> ATFISVQLKKTSEVDLAKPLVKFIQQTYPSGGEEQAQYCRAAEELSKLRRAAVGRPLDKHEGALETLLRYYDQICSIEPKFPFSENQICLTFTWKDAFDKGSLFGGSVKLALASLGYEKSCVLFNCAALASQIAAEQNLDNDEGLKIAAKHYQFASGAFLHIKETVLSALSREPTVDISPDTVGTLSLIMLAQAQEVFFLKATRDKMKDAIIAKLANQAADYFGDAFKQCQYKDTLPKEVFPVLAAKHCIMQANAEYHQSILAKQQYYFGEEIARLQHAAELIKTVASRYDEYVNVKDFSDKINRALAAAKKDNDFIYHDRVPDLKDLDPIGKATLVKSTPVNVPISQKFTDLFEKMVPVSVQQSLAAYNQRKADLVNRSIAQMREATTLANGVLASLNLPAAIEDVSGDTVPQSILTKSRSVIEQGGIQTVDQLIKELPELLQRNREILDESLRLLDEEEATDNDL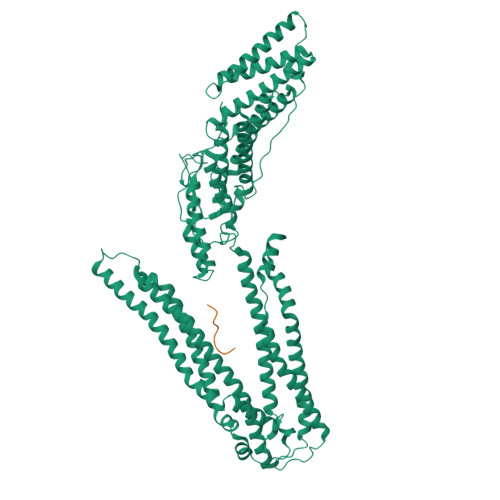RAKFKERWQRTPSNELYKPLRAEGTNFRTVLDKAVQADGQVKECYQSHRDTIVLLCKPEPELNAAIPSANPAKTMQGSEVVNVLKSLLSNLDEVKKEREGLENDLKSVNFDMTSKFLTALAQDGVINEEALSVTELDRVYGGLTTKVQESLKKQEGLLKNIQVSHQEFSKMKQSNNEANLREEVLKNLATAYDNFVELVANLKEGTKFYNELTEILVRFQNKCSDIVFAR;> NLYPDLSE Here, we identified the BBDE_2040 gene product from Bifidobacterium dentium (α-D-fructofuranosidase and difructose dianhydride I synthase/hydrolase from Bifidobacterium dentium [αFFase1]) as an enzyme with α-D-fructofuranosidase and α-D-arabinofuranosidase activities and an anomer-retaining manner. αFFase1 is not homologous with any known enzymes, suggesting that it is a member of a novel glycoside hydrolase family. αFFase1 did not catalyze any reactions when DFA III or inulin was used as a substrate, and there were no significant peak changes in the reaction of caramelized sugars other than those of the four peaks. These results indicate that αFFase1 specifically catalyzes the reversible hydrolysis of the intramolecular α-(2→1′)-D-fructofuranosidic bond of DFA I and DHL II. Because of the significant bias of equilibrium toward DFA synthesis, we propose a common name difructose dianhydride I synthase/hydrolase for this enzyme (EC 3.2.1.134). Each monomer consists of β-jelly roll 1 (residues 3–200, green), β-jelly roll 2 (201–396, magenta), and a 51-amino acid–long α-helix at the C terminus (397–448, blue), englobing the whole structure.

The ligand-free structure was determined at 1.96 Å resolution. The asymmetric unit contained a hexamer with D3 dihedral symmetry. The hexameric structure corresponded to the possible biological assembly that was implied by size-exclusion chromatography and the PISA server. The six chains in the asymmetric unit have virtually identical structures, as the average RMSD and their SD for the Cα atoms between all chain pairs are 0.15 ± 0.03 Å (maximum = 0.19 Å in 15 pairs). A Dali structural similarity search of the whole monomer showed that αFFase1 is similar to the hypothetical protein BACUNI_00161, which is used as a template for molecular replacement. Several capsid proteins of phages showed weak structural similarities (Z score >8). A metal ion was observed close to the active site (green sphere), although the buffers used during protein purification and crystallization contained no divalent metal ions. The metal ion in the crystal structure was assigned as Ca2+ based on the analysis using the CheckMyMetal server. Treatment with excess amount of EDTA did not inhibit the activity of αFFase1.

>MSEITGLFKDLTKVKHARNGRLASWDQRGKNQDYWEIPAGESITLGEIEGPGCITHMWMTSSCRKVVAPSILDPELNASAAPVMEIHPALGVIWDAYDPFYYRKALIKITWDDQDTPSVLVPFGDFFCIGNSYPGNFSSLPFNVSLKPEEAGKFGAPCSVSCYFPMPFNKKAKIEIVNDNELPFILYFNIDYEMYGEPLPEDTAYFHAAWHRENPCNGWGPELQVNSPEVNNVTNFKGENNYTVLDVEGTGHYVGCNLTVKHFQGSWWGEGNDMFFIDGEEYPSLNGTGTEDYFNHAWGMQRNAYPFFGTIVHEGDTDGFQVSYRWHITDPVRFEKHLKVTIEHGHANQLSDDWSSTAYWYQILPTASRITIAPVEDRLPVVPQLPERKLVLPQLTEEQQAARDTYQKRWKDYEPRRDTQFRIKEDKARRESKLNTEFAKKLRDAFDAEREQLEHHHHHH[6x]N-{(1R)-2-[(4-CYANO-1,1-DIOXIDOTETRAHYDRO-2H-THIOPYRAN-4-YL)AMINO]-2-OXO-1-[(TRIMETHYLSILYL)METHYL]ETHYL}MORPHOLINE-4-CARBOXAMIDE | C17 H30 N4 O5 S Si | 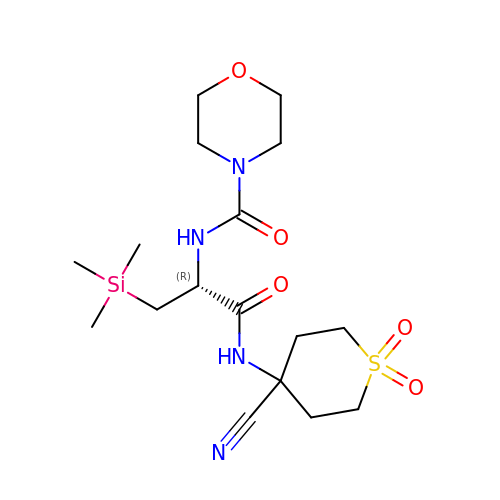VASVHRZIUGJLOH-AWEZNQCLSA-N> TPVSEKQLAEVVANTITPLMKAQSVPGMAVAVIYQGKPHYYTFGKADIAANKPVTPQ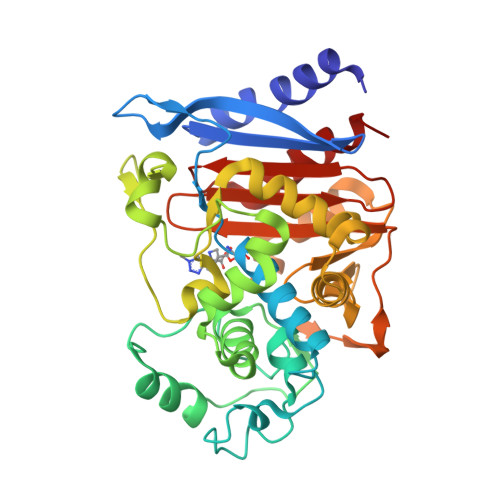TLFELGSISKTFTGVLGGDAIARGEISLDDPVTRYWPQLTGKQWQGIRMLDLATYTAGGLPLQVPDEVTDNASLVRFYQNWQPQWKPGTTRLYANASIGLFGALAVKPSGMPYEQAMTTRVLKPLKLDHTWINVPKAEEAHYAWGYRDGKAVRVSPGMLDAQAYGVKTNVQDMANWVMANMAPENVADASLKQGIALAQSRYWRIGSMYQGLGWEMLNWPVEANTVVEGSDSKVALAPLPVVEVNPPAPPVKASWVHKTGSTGGFGSYVAFIPEKQIGIVMLANTSYPNPARVEAAYHILEALQ> GPVDNNNNNGLKNSTEPIYAKVNKKKTGQVASPEEPIYTQVAKKVNAKIDRLNQIASGLGGVGQAAGFPLKRHDKVDDLSKVGLSASPEPIYATIDDL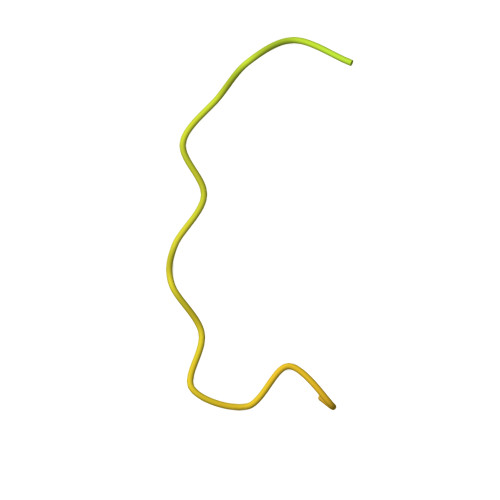GGPFPLKRHDKVDDLSKVGRSRNQELA(2R,3S,4R,5S)-2,6-difluoro-2-(hydroxymethyl)oxane-3,4,5-triol | C6 H10 F2 O5 | 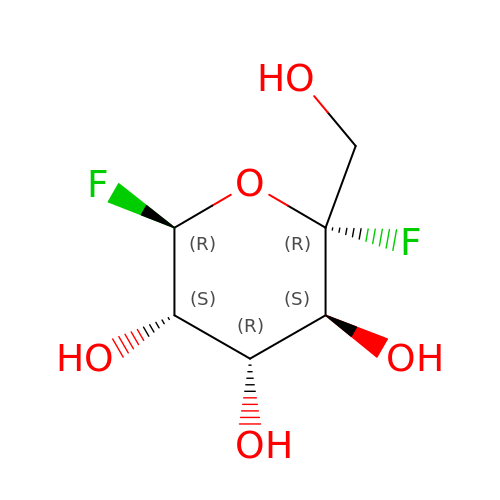MGHYRMVVRYCAON-NURPGYHYSA-N>DYKDDDDADTCGPCEPASCPPLPPLGCLLGETRDACGCCPMCARGEGEPCGGGGAGRGYCAPGMECVKSRKRRKGKAGAAAGGPGVSGVCVCKSRYPVCGSDGTTYPSGCQLRAASQRAESRGEKAITQVSKGTCEQGGSGGSSGGSGSGDTEAVVCVGTACYTAHSGKLSAAEAQNHCNQNGGNLATVKSKEEAQHVQRVLAQLLRREAALTARMSKFWIGLQREKGKCLDPSLPLKGFSWVGGGEDTPYSNWHKELRNSCISKRCVSLLLDLSQPLLPSRLPKWSEGPCGSPGSPGSNIEGFVCKFSFKGMCRPLALGGPGQVTYTTPFQTTSSSLEAVPFASAANVACGEGDKDETQSHYFLCKEKAPDVFDWGSSGPLCVSPKYGCNFNNGGCH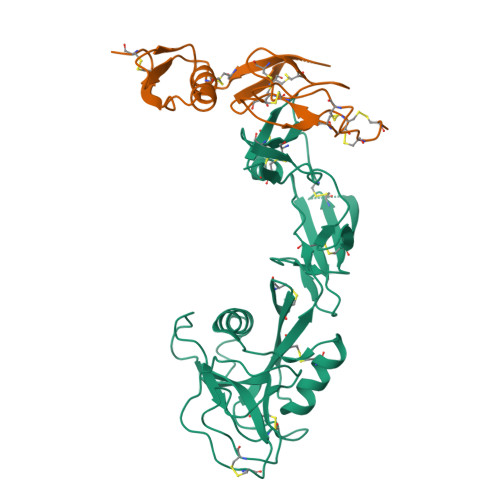QDCFEGGDGSFLCGCRPGFRLLDDLVTCASRNPCSSSPCRGGATCVLGPHGKNYTCRCPQGYQLDSSQLDCVDVDHHHHHHHA[4x]> MLGPKRCSMVLDVAFVLEGSDKIGEADFNRSKEFMEEVIQRMDVGQDSIHVTVLQYSYMVTVEYPFSEAQSKGDILQRVREIRYQGGNRTNTGLALRYLSDHSFLVSQGDREQAPALVYMVTGNPASDEIKR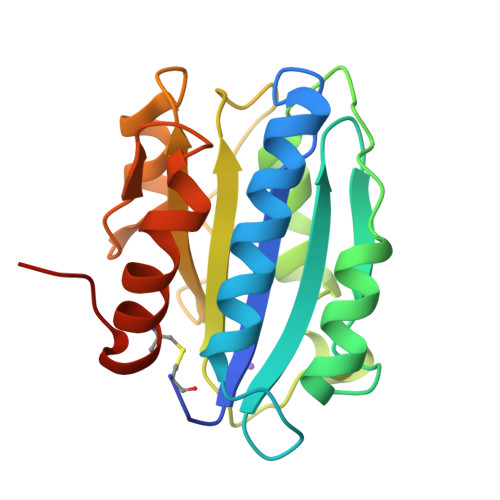LPGDIQVVPIGVGPNANVQELERIGWPNAPILIQDFETLPREAPDLVLQRCSSGEGLEHHHHHH> MVAKGRIIRVTGPLVVADGMKGAKMYEVVRVGELGLIGEIIRLEGDKAVIQVYEETAGVRPGEPVVGTGASLSVELGPGLLTSIYDGIQRPLEVIREKTGDFIARGVTAPALPRDKKWHFIPKAKVGDKVVGGDIIGEVPETSIIVHKIMVPPGIEGEIVEIAEEGDYTIEEVIAKVKTPSGEIKELKMYQRWPVRVKRPYKEKLPPEVPLITGQRVIDTFFPQA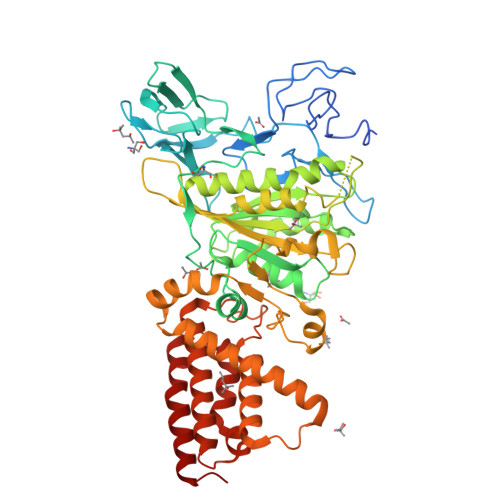KGGTAAIPGPFGSGKTVTQHQLAKWSDAQVVIYIGCGERGNEMTDVLEEFPKLKDPKTGKPLMERTVLIANTSNMPVAAREASIYTGITIAEYFRDMGYDVALMADSTSRWAEALREISGRLEEMPGEEGYPAYLASKLAEFYERAGRVVTLGSDYRVGSVSVIGAVSPPGGDFSEPVVQNTLRVVKVFWALDADLARRRHWPAINWLTSYSLYVDAVKDWWHKNIDPEWKAMRDKAMALLQKESELQEIVRIVGPDALPERERAILLVARMLREDYLQQDAFDEVDTYCPPEKQVTMMRVLLNFYDKTMEAINRGVPLEEIAKLPVREEIGRMKFERDVSKIRSLIDKTNEQFEELFKKYGA> SYVAHLASDFGVRVFQQVAQASKDRNVVFSPYGVASVLAMLQLTTGGETQQQIQAAMGFKIDDKGMAPALRHLYKELMGPWNKDEISTTDAIFVQRDLKLVQGFMPHFFRLFRSTVKQVDFSEVERARFIINDWVKTHTKGMISHLLGTGAVDQLTRLVLVNALYFNGQWKTPFPDSSTHRRLFHKSDGSTVSVPMMAQTNKFNYTEFTTPDGHYYDILELPYHGDTLSMFIAAPYEKEVPLSALTNILSAQLISHWKGNMTRLPRLLVLPKFSLETEVDLRKPLENLGMTDMFRQFQADFTSLSDQEPLHVALALQKVK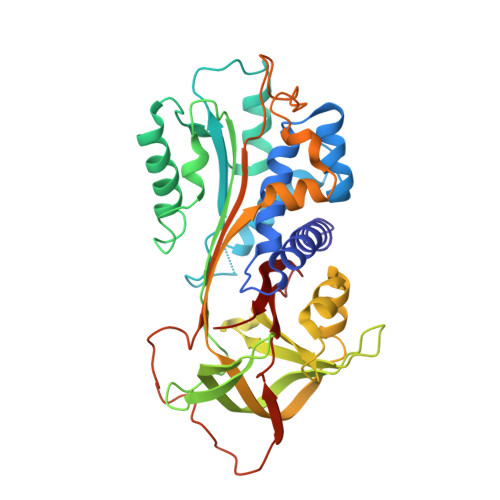IEVNESGTVASSSTAVIVSARMAPEEIIIDRPFLFVVRHNPTGTVLFMGQVMEP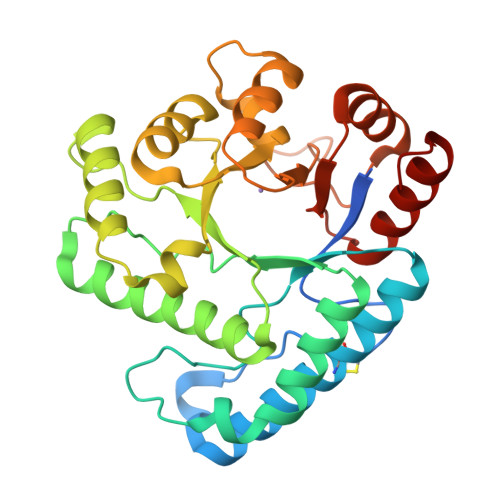>[2x]MGHHHHHHHHHHSSGHIEGRHMRVGYVSTNYSLGCKADKTIKLSSLSEERVLKVSSSNLLCLKNILEWNLKHEILFFRISSNTIPLASHPKFHVNWKDKLSHILGDIGDFIKENSIRISMHPGQYVVLNSVREEVVRSSIMELKYHADLLDSMGIEGKIQIHVGSSMNGKEESLNRFIENFRKLPSNISKRLVIENDDKVFSVKDCLWISERTGIPVIFDNLHHSILNNGESLNDALSLVRRTWKDRPMIDYSEQEPGEKPGVHATTINEENFRRFVNEVDEVDIMLEVKDKEISALKAVKVLKELNKLD> MSLSNRAGEILIVEDSPTQAEHLKHILEETGYQTEHVRNGREAVRFLSLTRPDLIISDVLMPEMDGYALCRWLKG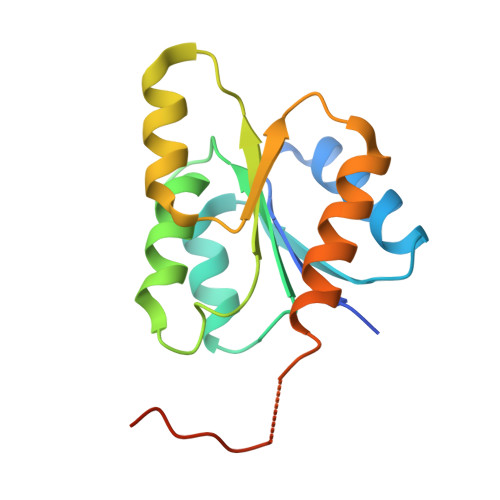QPDLRTIPVILLTILSDPRDVVRSLECGADDFITKPCKDVVLASHVKRLLSGVKRTEERYSRESITLAFGNEGHHHHHH>[4x]GSHMMPYLKGAPMNLQEMEKNSAKAVVLLKAMANERRLQILCMLLDNELSVGE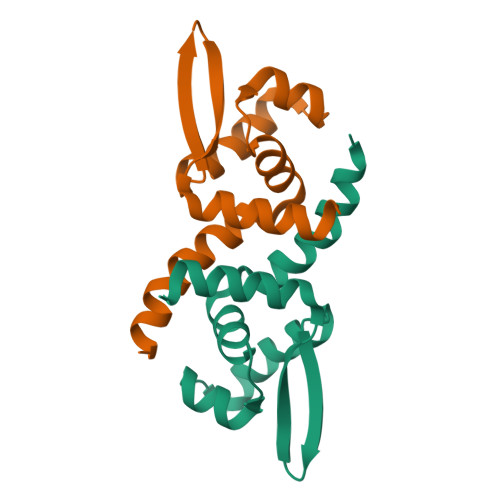LSSRLELSQSALSQHLAWLRRDGLVNTRKEAQTVFYTLSSTEVKAMIELLHRLYCQANQ> GLLSILRKLKSAPDQEVRILLLGLDNAGKTTLLKQLASEDISHITPTQGFNIKSVQSQGFKLNVWDIGGQRKIRPYWRSYFENTDILIYVIDSADRKRFEETGQELTELLEEEKLSCVPVLIFANKQDLLTAAPASEIAEGLNLHTIRDRVWQIQSCSALTGEGVQDGMNWVCKN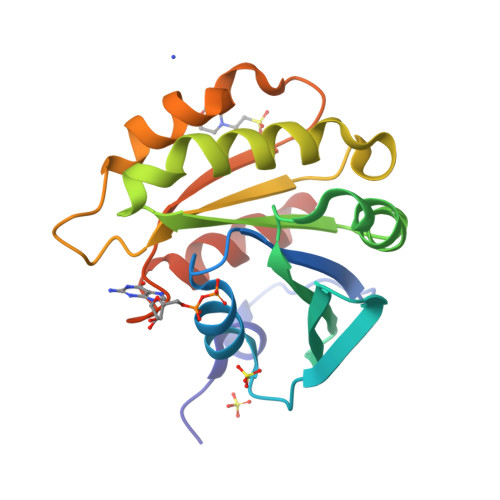VNAKKK> GSGLDDVSNKAYEDAEAKAKYEAEAAFFANLKLSDFNIIDTLGVGGFGRVELVQLKSEESKTFAMKILKKRH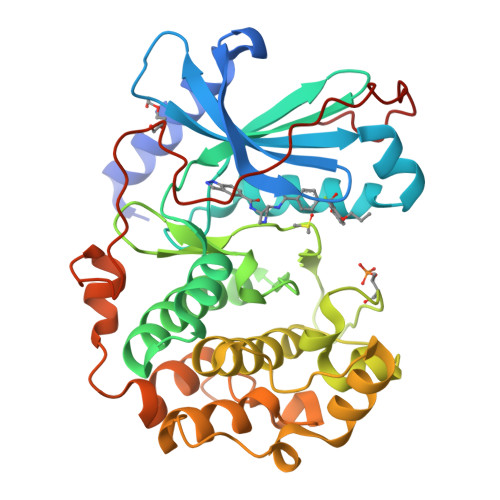IVDTRQQEHIRSEKQIMQGAHSDFIVRLYRTFKDSKYLYMLMEACLGGELWTILRDRGSFEDSTTRFYTACVVEAFAYLHSKGIIYRDLKPENLILDHRGYAKLVDFGFAKKIGFGKKTWTFCGTPEYVAPEIILNKGHDISADYWSLGILMYELLTGSPPFSGPDPMKTYNIILRGIDMIEFPKKIAKNAANLIKKLCRDNPSERLGNLKNGVKDIQKHKWFEGFNWEGLRKGTLTPPIIPSVASPTDTSNFDSFPEDNDEPPPDDNSGWDIDF>MKHHHHHHPMSDKIIHLTDDSFDTDVLKADGAILVDFWAEWCGPCKMIAPILDEIADEYQGKLTVAKLNIDQNPGTAPKYGIRGIPTLLLFKNGEVAATKVGALSKGQLKEFLDANLAGSAMESTVMVLRNMVDPKDIDDDLEGEVTEECGKFGAVNRVIIYQEKQGEEEDAEIIVKIFVEFSIASETHKAIQALNGRWFAGRKVVAEVYDQERFDNSDLSA[4x]

UHM-ULM interactions mediated by multiple ULMs of SF3b1 and UHM domains from SPF45, PUF60 and CAPER-α play a crucial role in AS. UHM domains were first identified in both subunits of the U2AF heterodimer (U2AF65 and U2AF35). Structural analysis revealed that they represent non-canonical RNA recognition motif (RRM) domains with degenerate RNA binding motifs. Using high-throughput screening (HTS) of a highly curated library of 43296 drug-like molecules with biophysical assays monitoring binding to UHM domains, we identified phenothiazine derivatives as inhibitors of UHM-ULM interactions.

To confirm the binding pose of the compound we pursued crystallization attempts with other UHM domains. This approach is based on the observation that the ULM-binding pockets of UHM domains are highly conserved suggesting that our small molecule inhibitors will bind to other UHM domains using a similar binding mode. The absence of electron density of the ligand in the other two molecules of the asymmetric unit results from the fact that the binding site is blocked by symmetry-mates in the crystal. As expected, the phenothiazine moiety of 7,8-dimethoxyperphenazine occupies the tryptophan-binding pocket. The binding pocket is slightly expanded compared to the recognition of ULM peptide in order to accommodate the three aromatic rings of the phenothiazine. The tricyclic ring system adopts a non-planar bent arrangement due to the presence of the sulfur heteroatom. The hexagonal ring attached to the 7,8-dimethoxy position forms π-stacking interaction with Phe534 of the UHM domain. The chlorine atom snuggly fits into the hydrophobic tryptophan-binding pocket of the UHM domain. The 7-methoxy group of the compound points to the pocket that is normally occupied by Arg337 of the ULM peptide ligand, whereas the 8-methoxy group is solvent exposed. The ion pair of the tertiary N14-amine group of the piperazine moiety interacts with the Glu483 sidechain, which in turn is stabilized via hydrogen bond with the side chain of Lys486.> AVPGYYELYRRSTIGNSLVDALDTLISDGRIEASLAMRVLETFDKVVAETLKDNTQSKLTVKGNLDTYGFCDDVWTFIVKNCQVTVEDSHRDASQNGSGDSQSVISVDKLRIVAC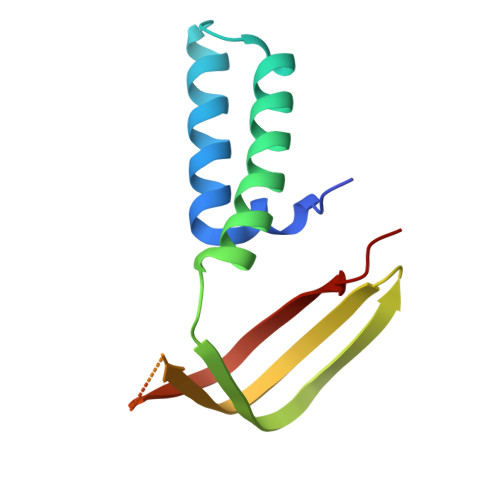NSKKSE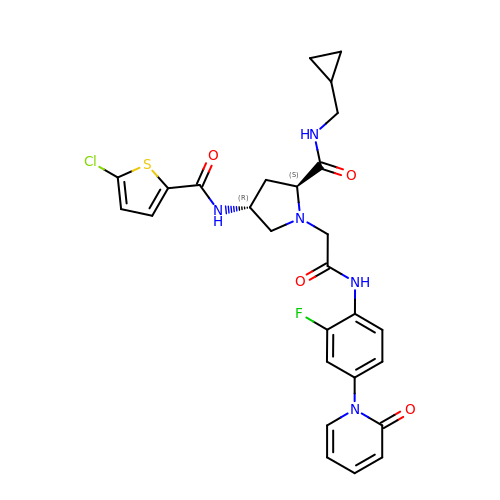(4R)-4-{[(5-chlorothiophen-2-yl)carbonyl]amino}-N-(cyclopropylmethyl)-1-(2-{[2-fluoro-4-(2-oxopyridin-1(2H)-yl)phenyl]amino}-2-oxoethyl)-L-prolinamide | C27 H27 Cl F N5 O4 S | LRFNMAKOTZSBFP-UTKZUKDTSA-N The bifunctional enzyme Δ1-pyrroline-5-carboxylate synthase (P5CS) is vital to the synthesis of proline and ornithine, playing an essential role in human health and agriculture. The P5CS molecule contains two domains, GK and GPR, catalyzing the first and second steps in the biosynthesis of proline from glutamate. The GK domain catalyzes glutamate phosphorylation, and the GPR domain catalyzes the NADPH-dependent reduction of γ-glutamyl phosphate (G5P) to glutamate-γ-semialdehyde (GSA). Our results describe the assembly mechanism of P5CS filaments, in which the GK domain forms tetramer and the GPR domain forms dimer structure, and both domains form specific interaction interfaces.

In the P5CSGlu filament, no ligand binds to the GPR domain. Conformational comparison of unliganded, G5P-binding and NADP(H)-released states shows that the overall structures of the GPR domain are similar. The structure of the NADP(H)-release state, which has no bound ligand, is identical to the unliganded state. In our models, unliganded, G5P-binding and NADP(H)-released states represent as open conformation, and the NADP(H)-binding state represents as closed conformation. The interaction formed between F642-P644 of the contact loops in adjacent GPR domains, which appears as a CH/Pi interaction, is critical for the filamentation. In the P5CSGlu filament, the GK and GPR domains are likely in a stable conformational state, while vibration may occur in the GPR domain of P5CSGlu/ATPγS and P5CSMix filaments due to the binding of ligands.

>MLQNSFKLAQSLRNGFYRNAWRAFSSHGPRQPLVSPERRLEKAHPTFTERSQLKYARRLVVKLGSAVITREDNHGLALGRLASIVEQVAECHLEGREVMMVTSGAVAFGKQKLAQELLMSLSMRETLNPKDSKEFDGATLEPRAAAAVGQSGLMSLYDAMFAQYGVKIAQVLVTKPDFYNEETRNNLFCTLSELISLNIVPIINTNDAVSPPMFIRDDEPAGGARRGIPIKDNDSLSAMLAAEVQADLLILMSDVDGIYNKPPWEDGAKLMHTYTSDDSNSIEFGKKSKVGTGGMDSKVKAATWALDRGVSVVICNGMQEKAIKTIIGGRKVGTFFTEATESANAVPVEVMAENARTGSRQMQALTPAQRASAVNTLADLLVSREKFILDANAKDLAEAQKSGLAKPLLSRLSLNPAKLKNLSVGLKQIAEDSHKNVGRVLRRTRLADQLELKQVTVPIGVLLVIFESRPDSLPQVAALAMASANGLLLKGGKEAAHSNKALMELVKEALATVGAEHAVSLVSTREEISDLLSMENHIDLIIPRGSSDLVRSIQQQSLHIPVLGHAEGVCHVYIDRDADLEKALRIARDAKCDYPAACNAMETLLIHEDLMSGAIFGDVCNMLKREGVKIYAGPRLNQQLTFGPPAAKSLKHEYGALECCIEVVPSLDEAINHIHTYGSSHTDVIVTENDAAARQFLGSVDSACVFHNASSRFADGFRFGLGAEVGISTARIHARGPVGVEGLLTTKWILEGQDHAAADFAEGGGRTWLHETLPLD[2x]> MRFRIRKCPKCGRYTLKEVCPVCGEKTKVAHPPRFSPEDPYGEYRRRWKREVLG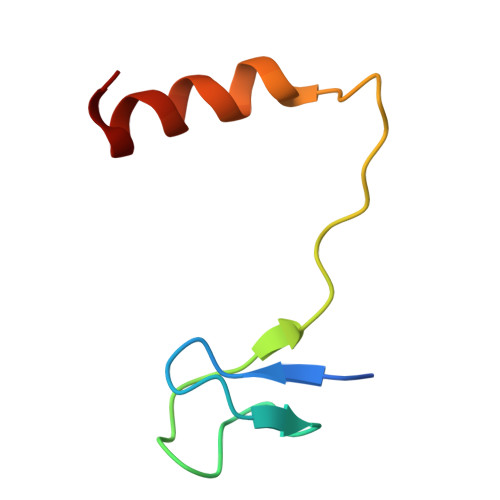I>SANLKNKTLVVTTILSNPYCMRKESAIPLSGNDQFEGYAVDLIHEISKSLGFNYKIQLVPDGSYGSLNKLTGEW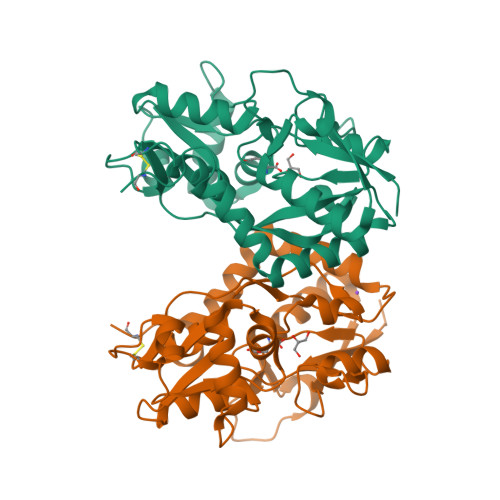NGMIRELLEQRADLAIADLTITFEREQAVDFTTPFMNLGVSILYRKGTPIESAEDLAKQTRIKYGALKGGSTAAFFRDSKISTYQRMWSFMESARPSVFTASNGEGVERVAKGKGSYAFLMESTSIEYVTERNCELTQVGGMLDTKSYGIATPPNSPYRTAINSVILKLQEEGKLHILKTKWWKEKRGGGKCR[2x]>PTAAEDLRHKKKRLTAMERVQLFCDPGTFRERDALVEHECHNFGMEKRKVPGDGFITGTGKVFGRPVFLFSHDFTVFGGSLSRTNAAKVVRIMEEAAKIGVPVIGFNDSGGARIHEGVDSLAGYADIFLRNTLFSGVIPQISVIMGPCAGGAVYSPAITDFTFMVETSSYMFVTGPEVVSAVGGKLVTKDELGGPHVHATKSGVSAGTFPNDIVAMAQLRRLYSYLPLSNRDPVPVLPTADERYRDVSSLNTVVPTEVKEAYDMRDVIYPVIDHDSFFEIQPQFAKNIICGFARVEGRSVCIIANQPKVQAGVLDIDSSVKGARMVRFADAFNIPIITFVDVPGFLPGVQQEYGGIIRHGAKLLYAYAEATVPKVTIITRKAYGGAYDVMSSKHLRGDSNYAWPHAEIAVMGAAGACKLLYSKETAEQQAQRIADYEKTFCTPLSAARKGFVDAVIDPSETRMRVCEDLERLARKQLQNPWKKHGNIPL[6x];>VLVANRGEIACRVMATCRRLGIKTVAVYSTADEQAKHVKVADESVCIGPPASVESYLCIDKIVDACKKTGAQAVHPGYGFLSENGEFQSALQKNNIVFVGPDAHSIESMGDKIESKRLAQRAGVTCIPGFIGEVKTHEDLLRFAREIGYPVMIKASGGGGGKGMRVAYNDTQCVEYYDMCREEAKAAFHSDKMLVERFIDHPRHIEIQVIADRRGNTVYLPERECSIQRRNQKVIEEAPSVLLDATTRKAMGEEAVAMARAVQYVSAGTVENVVNPQKQFYFLEMNTRLQVEHPITEEITGVDLVEQMLRAAADLPLSITQDDITINGHATECRVYAEDPMKNYFPSIGRLTMYQEPTGAGVRCDSGIIEGSQISVYYDPLICKLSTWGRDRAECIGRMEKALDEYVIRGLRHNICLLRDVVTEPRYRSGSITTNYLQEQYPNGFKKAELTAEEMQLMYEVAACVHLKRERLHYTQGTAPSERQLYLSVGAGQEGETPVYVRYLDDSHFEIGASKHGPFRKMEVVWKASYPIIRVKDGEAETVLQFWGTNEVTYGMQMRGTTFDVNVMSDLQSTLAHFVPITEATTNTKQILSPMPGVIVAIKVQPGQMVVAGEELLTLEAMKMRNKIHAQADGKVKEVKVKLGATVEDNEVLVELE[4x]

One such multienzyme is propionyl-CoA carboxylase (PCC), which catalyzes the carboxylation of propionyl-CoA to form methylmalonyl-CoA, a precursor to the citric acid cycle intermediate succinyl-CoA. Propionyl-CoA carboxylase (PCC) is a multienzyme complex consisting of up to six α-subunits and six β-subunits. The α-subunit of LtPCC contains three domains: a biotin carboxylase (BC) domain, BC-CT mediating (BT) domain, and biotin carboxyl carrier protein (BCCP) domain. The β-subunit is composed of the structurally homologous N-carboxyltransferase (N-CT) and C-carboxyltransferase (C-CT) domains (Huang et al., 2010, Scheffen et al., 2021).

Here, we report three structures of endogenous LtPCC: an α6β6 dodecamer, α5β6 undecamer, and α4β6 decamer. To sort out LtPCCs with missing α-subunits, we performed symmetry-relaxed 3D classification and determined two additional LtPCC structures: α5β6 undecamer, α4β6 decamer. The α5β6 undecamer lacks one α-subunit, and the α4β6 decamer lacks two α-subunits on opposite sides of the LtPCC complex. In our decamer, undecamer, and dodecamer, the conformation of individual subunits is preserved. In other words, the structures of these complexes differ from one another only in the number and positioning of α-subunits. For each oligomeric isomer, the α-β binding site is either occupied or unoccupied. There are sixteen possible different LtPCC oligomeric isomers represented by seven oligomeric formulae (one isomer for α6β6, α5β6, α1β6 and α0β6, and four for α4β6, α3β6 and α2β6). In other oligomeric isomers, at least one active site cannot participate in catalysis, and so all non-dodecameric PCCs are less catalytically active than the dodecamer. Therefore, we propose that β-homohexamers are stable in solution, and the lack of interactions between PCC α-subunits allow for a continuous assembly and disassembly of α-subunits from β-homohexamers.> TKGAIVRWGKRKEKLIEEIRAREEERNALVVRLGEIDRTFAVAREEFDTVVKELEEARKSLYEGEARIKRAEEEKERLKAEILTGEARLPGLRERAENLRRLVEEKRAEISELERRLSSIT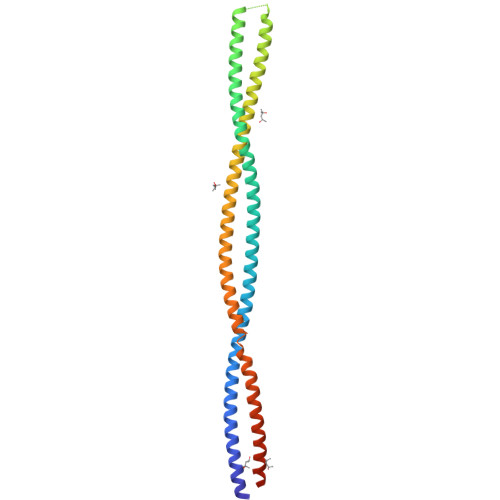SKRSGGSLESQSFELRIKLSDLEKELELARKDLEKVLAEERAVREEIEVAKRRINELDTLIERERGELAKLRGRIERLERKRDKLKKALENPEARELTEKIRAVEKEIAALREELSRVEGKLEGLESKVDAGSSSRPGL>GLEIMIGKKKGIQGHYNSCYLDSTLFCLFAFSSVLDTVLLRPKEKNDVEYYSETQELLRTEIVNPLRIYGYVCATKIMKLRKILEKVEAASGFTSEEKDPEEFLNILFHHILRVEPLLKIRSAGQKVQDCYFYQIFMEKNEKVGVPTIQQLLEWSFINSNLKFAEAPSCLIIQMPRFGKDFKLFKKIFPSLELNITDLLEDTPRQCRICGGLAMYECRECYDDPDISAGKIKQFCKTCNTQVHLHPKRLNHKYNPVSLPKDLPDWDWRHGCIPCQNMELFAVLCIETSHYVAFVKYGKDDSAWLFFDSMADRDGGQNGFNIPQVTPCP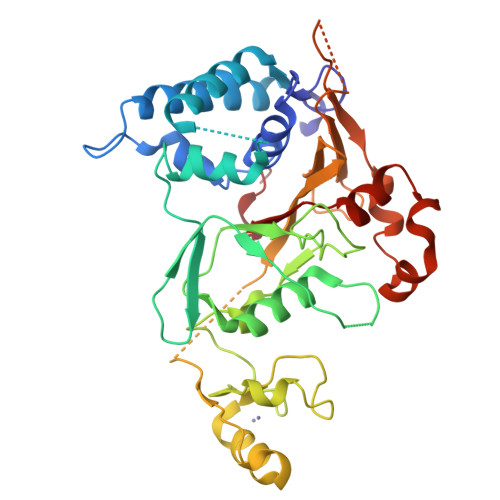EVGEYLKMSLEDLHSLDSRRIQGCARRLLCDAYMCMYQSPTMSLYK[2x]One of such splicing factors is polypyrimidine tract-binding protein 1 (PTBP1) which regulates a distinct set of splicing events by binding to polypyrimidine rich sequences found in introns. PTBP1 binds RNA through four RNA-recognition motifs (RRMs), that together recognize the polypyrimidine sequence for high affinity binding. A unique α3-helix is found in the linker between RRM1 and 2, which can be considered to be part of RRM1. By using a hydrocarbon peptide stapling approach, the helix could be mimicked to provide a peptide which can occupy its binding site and prevent PTBP1 from properly interacting with RNA.

To validate the interaction of the stapled peptides with RRM1 we attempted co-crystallization of either peptide P-2 or P-6 with RRM1Δα3. We observed crystals with the stitched peptide (P-6) in space group P21212 which diffracted to a resolution of 2.9 Å and had 16 dimers of protein–peptide complexes in the asymmetric unit (Fig. S7 and S8†). Also, we observed density of the hydrocarbon linkers between the unnatural amino acids which, like expected from the design, point away from the binding site. The placement of P-6 overlaps well with the original α3-helix and suggests the same hydrophobic binding core of I76, L80, V85, M90, and L88 on the RRM1 domain and A150, L152 and V154 on P-6. Additionally, polar interactions between E72 (RRM1) and R146 (P-6), the carbonyl oxygen of V85 (RRM1) and N155 (P-6), and side-chain–side-chain interactions of N87 (RRM1) and Q148 (P-6) are observed. No significant conformational changes were observed in RRM1 upon binding of our stapled peptides in comparison to the RNA-bound state (Fig. S10B†). However, the influence of P-6 competing with the native helix can't be observed with this protein structure, as the native α3-helix is not part of the protein construct used in this experiment. Since the peptide does not obscure the RNA-binding site of RRM1 we hypothesize that the stapled peptides block the correct orientation of both RRMs for high RNA affinity. To this end, we synthesized a set of hydrocarbon stapled peptides that mimic the helix and identified P-6 as a potent inhibitor of RNA-binding with a Ki of 9.3 μM.

>[16x]GPPSRVIHIRKLPIDVTEGEVISLGLPFGKVTNLLMLKGKNQAFIEMNTEEAANTMVNYYTSVTPVLRGQPIYIQFSNHKELKTDS;>NQLRAQXALQXVN[16x]>[2x]MHHHHHHSSGRENLYFQGPQDLMVTCTAPVNIAVIKYWGKRDEALILPINSSLSVTLHQDQLKTTTTVAISKDFTEDRIWLNGREEDVGQPRLQACLREIRRLARKRRSTEDGDTLPLSLSYKVHVASVNNFPTAAGLAS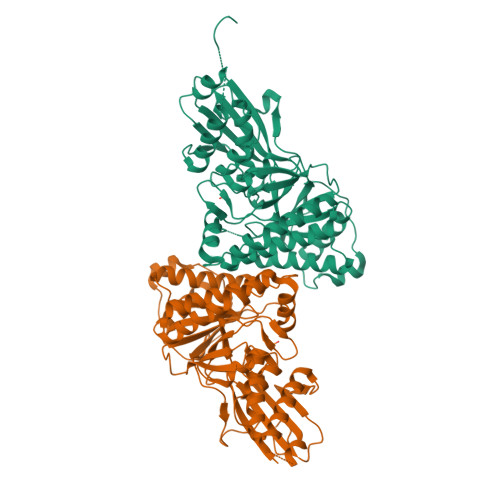SAAGYACLAYTLAQVYGVEGDLSEVARRGSGSACRSLYGGFVEWQMGEQADGKDSIARQIAPEWHWPQLRILILVVSADKKQTGSTVGMQTSVETSTLLKFRAESVVPERMKEMTRCIQEQDFQGFAQLTMKDSNQFHATCLDTFPPISYLNDTSRRIIQLVHRFNTHHGQTKVAYTFDAGPNAVIFTLEDTVAEFVAAVRHSFPPAANGDKFLKGLQVAPVLLSDELKAALVVEPSPGGVQYIIATQVGPGPQVLDDTHDHLLGQDGLPQRDL> PDVPKGCEGPCKVQSYEQRHDISHVGKVLCVSDVTRGNGLTHRVGKRFC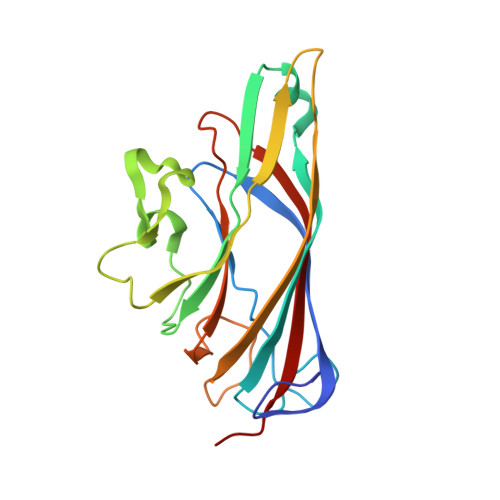VKSVYVLGKIWMDENIKTKNHTNTVMFYLVRDRRPFGTAMDFGQVFNMYDNEPSTATIKNDLRDRYQVLRKFTSTVTGGQYASKEQALVKKFMKINNYVVYNHQEAAKYDNHTENALLLYMACTHASNPVYATLKIRIYFYDSVQN> MSELYQAKSETRSTITSSLKGIQPYKPTKATIWSRADALKVNEYDPTTTQPLVSGDFPVMSDEVFIWNTMPLRDIDGNIASVNGWSVIFTLTADRNPTAPEYQDEQGNYDITLDWNDRHGRAKMYFWYSRTGKDWIIGGRVMAEGVSPTAREWA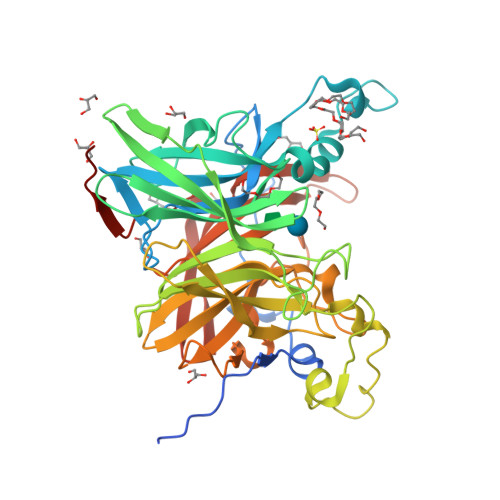GTPVLLNERGEIDLYYTAVTPGATVVKVRGRVVTTENGVEMVGFKKVKSLFEADGKMYQTESQNPYWAFRDPCPFRDPKSGKLYMLFEGNVAGERGSHVVGPDELGDVPPGYEDAGNSHFQTGCIGIAVCRDEDGDDWELLPPLITAVGVNDQTERPHFVFQDGKYYLFTISHKFTYGDGLTGPDGVYGFVSENLFGPYVPLNGSGLVLGNPPSQPYQTYSHYVMPNGLVTSFIDSVPTGEDSYRIGGTEAPTVLIKLKGAQTFVLEEFDYGYIPPMIDVKVEHHHHHH>MKTIGLLGGMSWESTIPYYRLINEGIKQRLGGLHSAQVLLHSVDFHEIEECQRRGEWDKTGDILAEAALGLQRAGAEGIVLCTNTMHKVADAIESRCTLPFLHIADATGRAITGAGMTRVALLGTRYTMEQDFYRGRL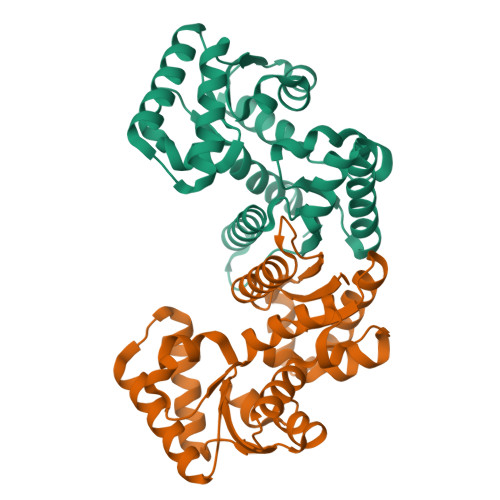TEQFSINCLIPEADERAKINQIIFEELCLGQFTEASRAYYAQVIARLAEQGAQGVIFGCTEIGLLVPEERSVLPVFDTAAIHAEDAVAFMLSLEHHHHHH[2x]> GSMKRSTTDSDLAGDAHNETNKKMKSTEEEEIGFSNLDENLVYEVL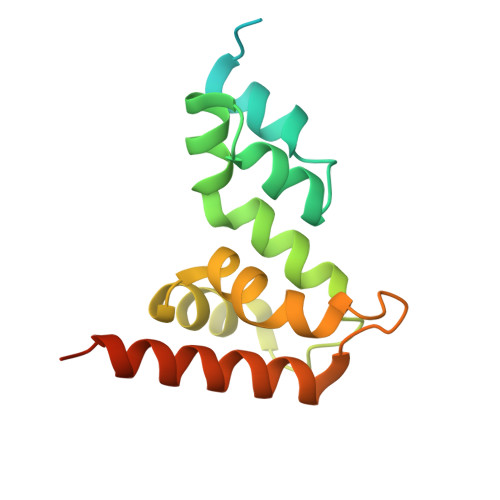KHVDAKTLAMSSCVSKIWHKTAQDERLWELICTRHWTNIGCGQNQLRSVVLALGGFRRLHSLYLWPLSKPNPRARFGKDELKLTLSLLSIRYYEKMSFTKRPLPESK Myophage Mu is a representative of contractile nanomachines with a simple tail baseplate. It has the capacity to infect a range of intestinal bacteria and has extensive applications in genetic engineering research. Using cryo-EM, we resolved the three-dimensional (3D) structures of the G(+) type phage Mu in both its extended state and urea-induced contracted state, the latter lacking the baseplate, at near-atomic resolutions. The structure of extended Mu can be divided into four distinct regions: the DNA-containing head, the connector complex, the tail, and the baseplate.

The absence of baseplate density in the contracted tail indicates that the baseplate may have detached during the process of tail contraction, potentially due to the effects of excessive urea induction. The terminator protein gp37 remains unaltered in both states, with the exception of the C-terminal β-hairpin domain. Upon contraction, the flexible C-terminal β-hairpin domain of gp37 elongates in conjunction with the domain I of the last layer of the tail sheath protein gp39, thereby accommodating sheath expansion. In the tail, the tube protein gp40 does not undergo any conformational change. However, the sheath protein gp39 undergoes significant conformational changes in both states. A structural comparison of the extended and contracted sheath monomers reveals that the N- and C-terminal arms of gp39 undergo significant conformational changes, indicating that each gp39 monomer primarily undergoes a rigid-body rotation, mediated by its N- and C-terminal arms, upon contraction. The contracted sheath retains the four-stranded β-sheet arrangement of all gp39 monomers, but the helical rise decreases from approximately 35 Å to approximately 19 Å, and the helical twist increases from approximately 25° to approximately 33°. The outer diameter of the sheath ring increases from 195 Å to 260 Å, and the inner pore diameter expands from 79 Å to 92 Å, which is sufficient to break the contacts between the tail sheath and tube. This process enables the sheath to be detached from the tube, resulting in the sheath becoming more compact and contracting, and the tail tube becoming exposed.

>MLEETEAALLARVRELFGATLRQVEPLTGTWTNEDVHRLFLAPPSVFLAWMGCGEGRTRREVESRWAFFVVAELLNGEPVNRPGIYQIVERLIAGVNGQTFGPTTGMRLTQVRNLCDDNRINAGVVLYGVLFSGTTPLPSVVDLDSLDDYERHWQTWKFPDETPEFAAHINVNQEKDHDAEN[6x];>MSDISFNAIPSDVRVPLTYIEFDNSNAVSGTPAPRQRVLMFGQSGSKASAAPNVPVRIRSGSQASAAFGQGSMLALMADAFLNANRVAELWCIPQGNGTGNAAVGEISLSGTAGENGSLVTYIAGQRLAVSVAAGATGAALADLLVARIKGQPDLPVTAEVRADSGDDDTHADVVLSAKFTGALSAVDVRWNYYAGETTPYGIITAFKAASGKNGNPDISASIAGMGDLQYKYIVMPYTDEPNLNLLRTELQERWGPVNQADGFAVTVLSGTYGDISTFGVSRNDHLISCMGIAGAPEPSYLYAATLCAVASQALSIDPARPLQTLTLPGRMPPAVGDRFTWSERNALLFDGISTFNVNDGGEMQIERMITMYRTNKYGDSDPSYLNVNTIATLSYLRYSLRTRITQKFPNYKLASDGTRFATGQAVVTPSVIKTELLALFEEWENAGLVEDFDTFKEELYVARNKDDKDRLDVLCGPNLINQFRIFAAQVQFIL[12x];>MAGNQRQGVAFIRVNGMELESMEGASFTPSGITREEVTGSRVYGWKGKPRAAKVECKIPGGGPIGLDEIIDWENITVEFQADTGETWMLANAWQADEPKNDGGEISLVLMAKQSKRIA[12x]> MATLSLTVNSGDPPLGALLAVEHVKDD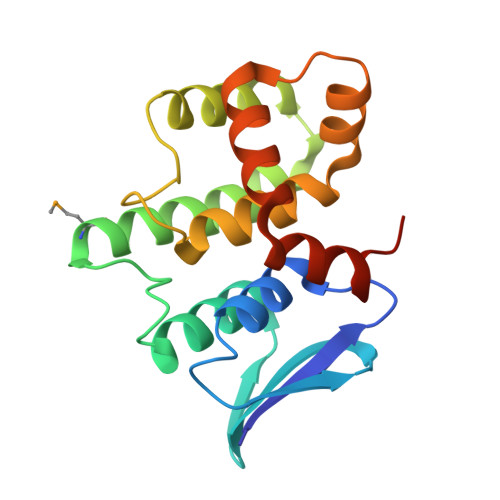VSISVEEGKENILHVSENVIFTDVNSILRYLARVATTAGLYGSNLMEHTEIDHWLEFSATKLSSSDSFTSTINELNHSLSLRTYLVGNSLSLADLSVWATLKGNAAWQEQLKQKKAPVHVKRWFGFLEAQQAFQSVGTKWDVSTTKAR The proteins involved are known and well-characterized. This includes the SNARE (Soluble N-ethylmaleimide−sensitive factor attachment protein receptor) proteins (VAMP2, Syntaxin, and SNAP25) that catalyze synaptic vesicle (SV) fusion, as well as chaperones Munc13, Munc18, and regulators Complexin and Synaptotagmin1–4. Syt-1 is anchored in the SV by a transmembrane domain (TMD), which is connected to tandem cytosolic C2 domains (C2A & C2B) via a 60-residue flexible linker. Both C2 domains are eight stranded anti-parallel beta sandwiches with one calcium sensing region consisting of two aliphatic loops containing Aspartic acid (Asp) residues that bind Ca2+16–18 These conserved Asp residues coordinate Ca2+ with the acidic lipids, like phosphatidylserine (PS) and phosphatidylinositol 4, 5-bisphosphate (PIP2), to facilitate the membrane insertion of the flanking aliphatic loops. In addition, the C2B domain has a conserved poly-lysine motif that binds to PS/PIP2 headgroups to mediate Ca2+-independent membrane interaction.

Using cryo-electron microscopy (Cryo-EM), we obtained 10 Å resolution reconstruction of the Syt1–SNARE complex on lipid membranes in the presence of Mg2+. This structure, derived from a helical crystal formed by covalently linked Syt1–SNARE protein applied to lipid tube surface, reveals that the Syt1 C2B domain concurrently binds both the SNARE proteins and the negatively charged membranes on diametrically opposite surfaces. So, we used a protein construct wherein the minimal C2AB domains of Syt1 (Syt1C2AB) are covalently linked to the SNARE complex, which was proven to be successful in 3D crystal formation. The optimum composition was found to be DOPS: GalCer at 80:20 ratio, which vastly improved both the overall frequency and quality of the helically organized Syt1C2AB-SNARE coated tubes. Helical indexing of the representative tube defined the Syt1C2AB-SNARE arrangement on the surface as 14,−4 start helix with a helical rise (Δz) of 7.35 Å and a helical twist (Δφ) of 78.48°. The resulting 3D reconstruction at 10.4 Å resolution showed protein decoration on the tube surface with prominent rod-like features (SNARE proteins) arranged almost parallel to the tube axis and with globular structures (C2 domains) attached to the membrane surface. The crystal structures were unambiguously docked into the EM map and showed SNAREpins arranged in an antiparallel fashion with membrane-distal C-terminal interaction. The Syt1 protein located between the SNARE complex and membrane surface, with the C2B domain interacting with the middle portion of SNARE complex. Relative position of C2B over the SNAREs was very similar to the recently described ‘primary’ binding site, involving the t-SNARE helices. The linker between the C2A and C2B domains was fully extended, with the C2A domain locating close to but not interacting with the N-terminal end of the same SNAREpin.

>[2x]KLGKLQYSLDYDFQNNQLLVGIIQAAELPALDMGGTSDPYVKVFLLPDKKKKFETKVHRKTLNPVFNEQFTFKVPYSELGGKTLVMAVYDFDRFSKHDIIGEFKVPMNTVDFGHVTEEWRDLQSAEK;>[4x]KLGKLQYSLDYDFQNNQLLVGIIQAAELPALDMGGTSDPYVKVFLLPDKKKKFETKVHRKTLNPVFNEQFTFKVPYSELGGKTLVMAVYDFDRFSKHDIIGEFKVPMNTVDFGHVTEEWRDLQSAEKEEQEKLGDICFSLRYVPTAGKLTVVILEAKNLKKMDVGGLSDPYVKIHLMQNGKRLKKKKTTIKKNTLNPYYNESFSFEVPFEQIQKVQVVVTVLDYDKIGKNDAIGKVFVGYNSTGAELRHWSDMLANPRRPIAQWHTLQVEEEVDAMLAVKK;>GSNRRLQQTQAQVDEVVDIMRVNVDKVLERDQKLSELDDRADALQAGASQFETSAAKLKRKYW[6x];>MALSEIETRHSEIIKLENSIRELHDMFMDMAMLVESQGEMIDRIEYNVEHAVDYVERAVSDTKKAVK[6x];>[6x]MRNELEEMQRRADQLADESLESTRRMLQLVEESKDAGIRTLVMLDEQGEQLDRVEEGMNHINQDMKEAEKNLKDLGK;>[6x]MARENEMDENLEQVSGIIGNLRHMALDMGNEIDTQNRQIDRIMEKADSNKTRIDEANQRATKMLG> VKYVVPSFSAGGLVQAMVTYEGDRNESAVFVAIRNRLHVLGPDLKSVQSLATGPAGDPGCQTCAACGPGPHGPPGDTDTKVLVLDPALPALVSCGSSLQGRCFLHDLEPQGTAVHLAAPACLFSAHHNRPDDCPDCVASPLGTRVTVVEQGQASYFYVASSLDAAVAASFSPRSVSIRRLKADASGFAPGFVALSVLPKHLVSYSIEYVHSFHTGAFVYFLTVQPASVTDDPSALHTRLARLSATEPELGDYRELVLDCRFAPKLVPRGSPEGGQPYPVLQVAHSAPVGAQLATELSIAEGQEVLFGVFVTGKDGGPGVGPNSVVCAFPIDLLDTLIDEGVERCCESPVHPGLRRGLDFFQSPSFCPNPPGLEALSPNTSCRHFPLLVSSSFSRVDLFNGLLGPVQVTALYVTRLDNVTVAHMGTM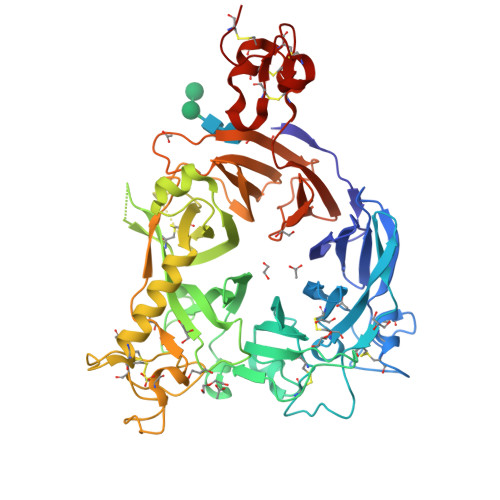DGRILQVELVRSLNYLLYVSNFSLGDSGQPVQRDVSRLGDHLLFASGDQVFQVPIQGPGCRHFLTCGRCLRAWHFMGCGWCGNMCGQQKECPGSWQQDHCP Wild-type streptavidin is a tetrameric protein with four identical subunits. Each subunit has a biotin binding pocket and can bind biotin tightly with a dissociation constant (Kd) around 10−14 M. This binding is considered to be irreversible and has been applied in a wide range of biomedical and biotechnological applications. Each streptavidin subunit contains eight antiparallel strands that form a β-barrel structure. Although each subunit can bind a biotin molecule, each of the four complete biotin pockets in the tetramer relies on the donation of Trp-120 located in loop from the neighboring subunit (e.g. subunit A needs Trp-120 from subunit D and vice versa).

A second approach is to create a mobile 8-amino-acid-loop (8-aa-loop) mutein in which loop is engineered to have a completely different sequence but retains the same length as the original loop in wild-type streptavidin. To avoid this complication, the H127C mutation was introduced to two constructs (8-aa-loop mutein and ΔW120 mutein) to create 8-aa-loop-H127C mutein and ΔW120-H127C mutein, respectively. The mutein with the lowest biotin binding affinity (1.9×10−8 M) in this study is the 8-aa-loop-H127C mutein. To assess the conformation of the 8-aa-loop-H127C mutein, the protein was crystallized in the presence of biotin and its structure was solved using X-ray crystallography. Using data extending to 2.0 Å resolution, the structure clearly shows that the mutein crystallizes as a tetramer with a single subunit in the asymmetric unit. Biotin is bound in a manner indistinguishable from that of wild-type streptavidin, but there is very little electron density for loop (residues 114–121) and its neighboring residue 113. The lack of electron density suggests that the modified sequence of loop confers a significant degree of dynamic disorder to the loop. In this case, the loss of order in loop of 8-aa-loop-H127C mutein allows for a much larger rearrangement of the A/B dimer relative to the C/D dimer. When the A/B dimer of the mutein is superimposed onto the A/B dimer of wild-type streptavidin, the C/D dimer is rotated by 11° relative to the position of the C/D dimer in wild-type streptavidin. An interesting feature also clearly seen in the crystal structure of the 8-aa-loop-H127C mutein is that a disulfide bond is formed between the Cys-127 residues of adjacent subunits at the A/B and C/D dimer interfaces.

> DPSKDSKAQVSAAEAGITGTWYNQLGSTFIVTAGADGALTGTYESAVGNAESRYVLTGRYDSAPATDGSGTALGWTVAWKNNYRNAHSATTWSGQYVGGAEARINTQWLLTSGDSSNGSDGSTLVGCDTFTKVKPSAASIDAAKKAGVNNGNPLDAVQQ>[4x]HMDKLPNIVILATGGTIAGSAATGTQTTGYKAGALGVDTLINAVPEVKKLANVKGEQFSNMASQNMTGDVVLKLSQRVNELLARDDVDGVVITHGTDTVEESAYFLHLTVKSDKPVVFVAAMRPATAISADGPMNLLEAVRVAGDKQSRGRGVMVVLNDRIGSARYITKTNASTLDTFKANEEGYLGVIIGNRIYYQNRIDKLHTTRSVFDVRGLTSLPKVDILYGYQD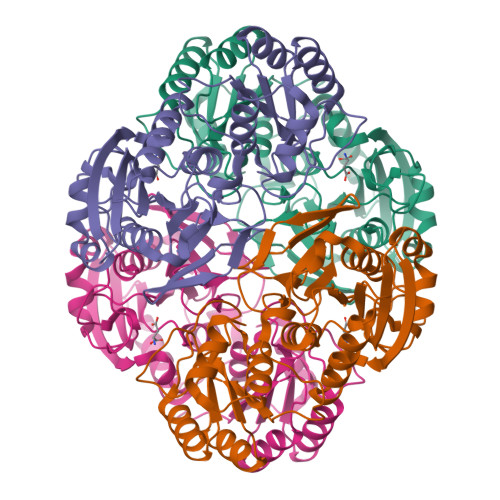DPEYLYDAAIQHGVKGIVYAGMGAGSVSVRGIAGMRKAMEKGVVVIRSTRTGNGIVPPDEELPGLVSDSLNPAHARILLMLALTRTSDPKVIQEYFHTY>[2x]MLSVENKVVAPPMVYIAGEEMTRYACDLVVKSWLEPYFDLSQWEYFDLSCVNRDNTNDQVLRDAVTAGQRIGAIFKEPTITPSAIQKKAFGLKNSLGSPNGAMRAGWNGITISRDTIHIDGIELGYKRPVFFERHAVGGEYGAGWSKVGRGTLLTTYLP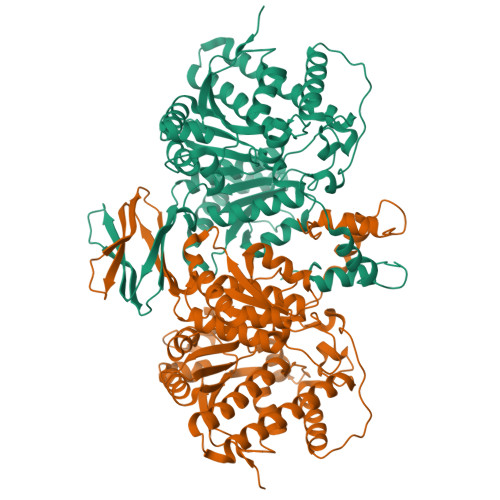SDGRDPFVVDKRDLTDQHNVVVTYHNPYDNVEPLAHLFFQRCLDANITPYVVTKKTVFKWQEGFWAVMKDVFDEHYKSRFEEKGLLQACGGDLQHLISDAATMQLIRWTDGGFGMAAHNYDGDMLTDQIAQVHRSPGFITSNLVGKAPDGSLIKEFEASHGTVSDLWNDHLAGKETSLNPLGLVEAIVGALQHAAVLDAEKNPDDEHKVKARDQIFNFTTTLRTAMHNTFRYGQGTRDMSGPSGYTTEDFVRKVAWRLQRYLDAQYDEAPPPQLGEPSRKLRRNYDIDEEAINGLFQKYDKNGDGFIDFEEFTRMLVKMNLAPLLTKKEKEKKPDV>[2x]MDTAGDTKTTDDGGVVNITYMHRLPDSEGMTLVNDIVAKWNKQHPDIQVKATKFDGKASDMIKKLETDVKSGEAPDLAQVGYAELPEVFTKGLLQDVTQYAEQYKNDFASGPYSLVQVGGKAYGLPQDTGPLVYFYNKAEFEK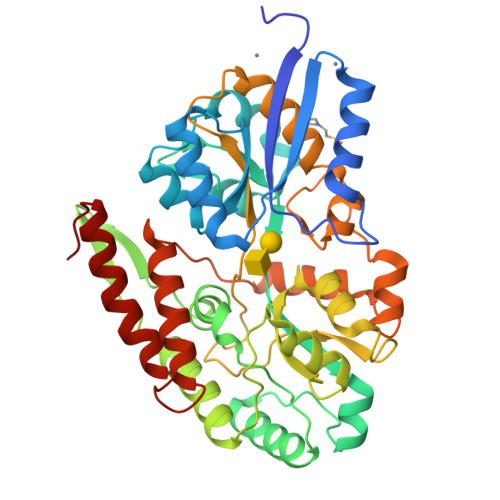LGITEIPQTADEFIAAAKTAAAAGKYIMSYQPDEAGNMISGLAGASGGWYKVKGDSWVVNTETDGSKATADFYQQLLDAKAATTNPRWDPSFDASIKDGSLIGTVAAAWEAPLFMTSSGGTGSGEWQVAQLGDWFGNAGKTGPDGGSAVAVLKNSKHPKEAMEFLDWFNTQVPDLVSQGLVPAATTEDAETPSEWSTFFGGQDIMKEFKTANNNMGDFTYMPGFSAVAAKMNETAAKATDGSGKVADIFSDAQTTSVDTLKNFGLSVSE> NAKNKESPTKAIVRLREHINLLSKKQSHLRTQITNQENEARIFLTKGNKVMAKNALKKKKTIEQLLSKVEGTMESMEQQLFSIESANLNLETMRAMQEGAKAMKTIHSGLDIDKVDET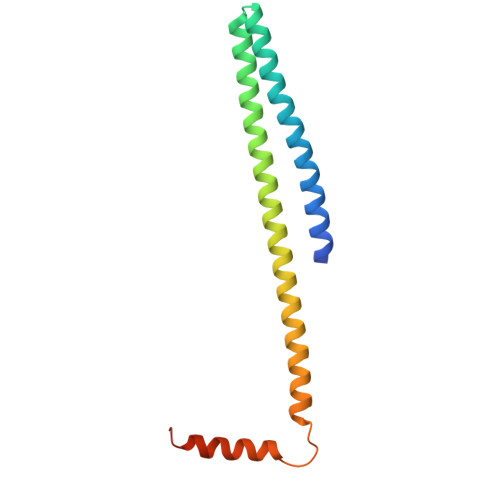MDEIREQVELGDEISDAISRP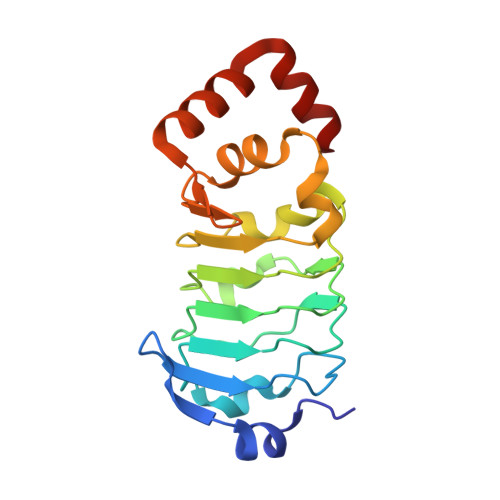> MVKLTPELINQSMQYINPVRERELDLRGYKIPQIENLGATLDQFDTIDLSDNDLRKLDNLPHLPRLKTLLLNNNRILRISEGLEEAVPNLGSIILTGNNLQELSDLEPLVGFTKLETISLLINPVSTKPNYREYMAYKFPQLRLLDFRKIKQKDRQAAQEFFRTKQGKDVLKEISR> MLKGFTPWPDELAETYRKNGCWAGETFGDLLRDRAAKYGDRIAITCGNTHWSYRELDTRADRLAAGFQKLGIQQKDRVVVQLPNIKEFFEVIFALFRLGALPVFALPSHRSSEITYFCEFAEAAAYIIPDAYSGFDYRSLARQVQSKLPTLKNIIVAGEAEEFLPLEDLHTEPVKLPEVKSSD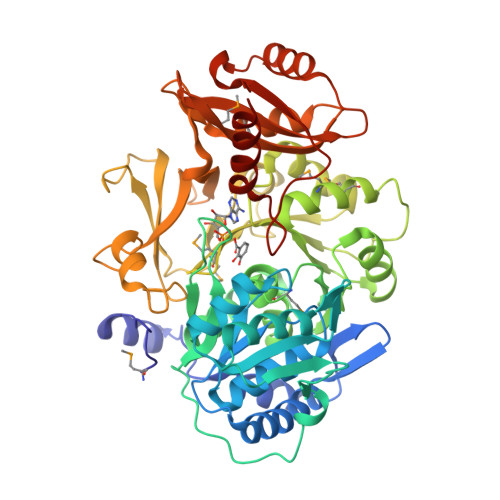VAFLQLSGGSTGLSKLIPRTHDDYIYSLKRSVEVCWLDHSTVYLAALPMAHNYPLSSPGVLGVLYAGGRVVLSPSPSPDDAFPLIEREKVTITALVPPLAMVWMDAASSRRDDLSSLQVLQVGGAKFSAEAARRVKAVFGCTLQQVFGMAEGLVNYTRLDDPEEIIVNTQGKPMSPYDESRVWDDHDRDVKPGETGHLLTRGPYTIRGYYKAEEHNAASFTEDGFYRTGDIVRLTRDGYIVVEGRAKDQINRGGEKVAAEEVENHLLAHPAVHDAAMVSMPDQFLGERSCVFIIPRDEAPKAAELKAFLRERGLAAYKIPDRVEFVESFPQTGVGKVSKKALREAISEKLLAGFKK> MVSVINTVDTSHEDMIHDAQMDYYGIRLATCSSDRSVKIFDVKNGGQILIADLRGHDGPVWQVAWAHPMYGNILASCSYDRKVIIWKEENGTWEKTYEYTGHDSSVNSVCWAPHDFGLVLACGSSDGAISILTFTGDGPWEVKKISNAHTIGCNAVSWAPSVIPGSLVDQPSSQKP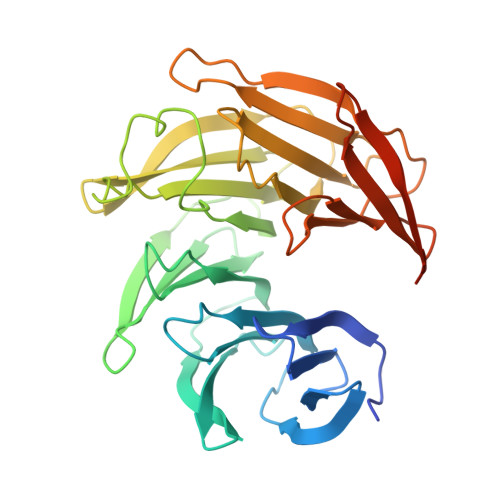NYIKRFVSGGCDNLVKIWREEDGQWKEDQKLEAHSDWVRDVAWAPSIGLPTSTIASCSQDGRVYIWTSDDAATNCWTPKLLHKFNDVVWHVSWSITANILAVSGGDNKVTLWKESVDGQWACISDVNKGQGAVSTVTEGQLNDQ> MSKAMALRRLMKEYKELTENGPDGITAGPSNEDDFFTWDCLIQGPDGTPFEGGLYPATLKFPSDYPLGPPTLKFECEFFHPNVYKDGTVCISILHAPGDDPNMYESSSERWSPVQSVEKILLSVMSMLAEPNDESGANIDACKMWREDREEYCRVVRRLARKTLGLLVPR;> GSHMLSSRISSSDNSSSSTGNEEVRNRSKLPSSKKEREELFRKRKEEMILAARKRMEGKIKGEKQDKN

Cells protect against this through pathways that include ER-associated degradation (ERAD), a process in which incorrectly folded proteins are ubiquitylated, marking them for extraction and subsequent degradation by the proteasome. ERAD requires specific E2 and E3 enzymes, including a conserved soluble E2: UBE2G2 (humans) or Ubc7 (Saccharomyces cerevisiae). These E2s are recruited to the ER by membrane-embedded proteins. Here, we identify the putative E2BR domain in S. pombe Cue4 and present a 1.7 Å resolution co-crystal structure of this E2BR in complex with S. pombe Ubc7.

The peak was pooled, concentrated and subjected to sparse-matrix crystallization screening. After refining the crystallization conditions, a crystal was grown that diffracted to 1.7 Å resolution in space group P212121 with a single complex in the asymmetric unit. The C-terminal end of S. pombe U7BR continues as a helix until residue 213, making it the longest contiguous helix of the three E2BRs. Human G2BR and S. pombe U7BR diverge at residue 180 of S. pombe U7BR (residue 574 of G2BR), where human G2BR ends and S. pombe U7BR turns towards the H2 face of Ubc7, forming a seven-residue N-terminal extension that lies on top of the H1 helix of Ubc7 and is unique among the three E2BRs. While the H. sapiens and S. cerevisiae E2BR domains used for crystallization were mostly ordered, with only a few residues at the N-terminus of G2BR that did not have sufficient density to be modeled, the longer S. pombe U7BR construct used for crystallization had 22 N-terminal residues that were not observed in electron density. The S. pombe Ubc7–U7BR complex buries a surface area of 2423 Å2 between the E2 and U7BR, as calculated using CNS. Three S. pombe U7BR residues that interact with Ubc7 are structurally and genetically conserved in the two other species: Lys192, Ala199 and Arg200. Superposition of E2–E2BR crystal structures on the structure of a cross-linked Ub E1–E2 complex reveals potential steric clashes between the N-termini of H. sapiens G2BR or S. pombe U7BR and the Ub-fold domain (UFD) of the Ub E1. While S. pombe U7BR appears to interfere with E1–Ubc7 binding, it presents no obvious structural impediment to Ubc7–E3 RING domain binding.> GPELVMRRGEIWQVSLGAARGAEANNQRPAVVVSNDRANATATRLGRGVITVVPVTSNIAKVYPFQVLLSATTTGLQVDCKA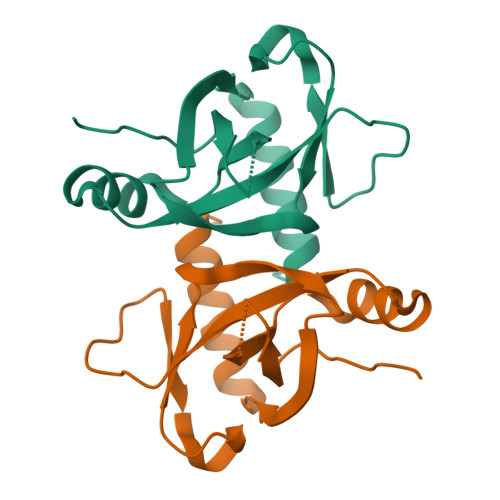QAEQIRSIATAALLRPIGRVSAAELAQLDEALKLHLDLWS> SSESTTFIVDVSPSMMKNNNVSKSMAYLEYTLLNKSKKSRKTDWISCYLANCPVSENSQEIPNVFQIQSFLAPVTTTATIGFIKRLKQYCDQHSHDSSNEGLQSMIQCLLVVSLDIKQQFQARKILKQIVVFTDNLDDLDITDEEIDLLTEELSTRIILIDCGKDTQEERKKSNWLKL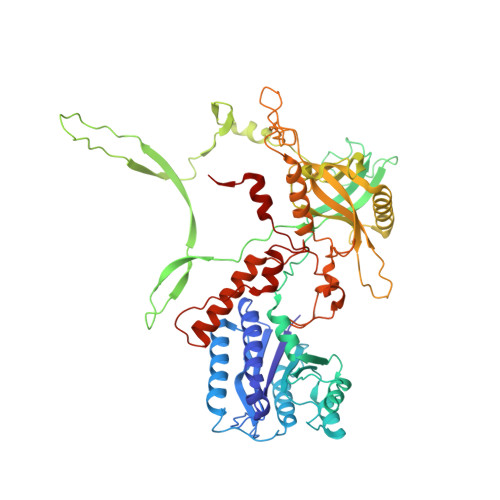VEAIPNSRIYNMNELLVEITSPATSVVKPVRVFSGELRLGADILSTQTSNPSGSMQDENCLCIKVEAFPATKAVSGLNRKTAVEVEDSQKKERYVGVKSIIEYEIHNEGNKKNVSEDDQSGSSYIPVTISKDSVTKAYRYGADYVVLPSVLVDQTVYESFPGLDLRGFLNREALPRYFLTSESSFITADTRLGCQSDLMAFSALVDVMLENRKIAVARYVSKKDSEVNMCALCPVLIEHSNINSEKKFVKSLTLCRLPFAEDERVTDFPKLLDRTTTSGVPLKKETDGHQIDELMEQFVDSMDTDELPEIPLGNYYQPIGEVTTDTTLPLPSLNKDQEENKKDPLRIPTVFVYRQQQVLLEWIHQLMINDSREFEIPELPDSLKNKISPYTHKKFDSTKLVEVLGIKKV>GSHMAKKPTIFILNGPNLNLLGLREPTIYGHQTLEDIANKLKLQAEKLDVTVEIRQSNHEGALIDWLQEAQAVKAKAVILNAAAYTHTSVAIYDAIRAITVPVIEVHLSNPHAREAFRHKSYVGEAALGTISGFGAESYSLALDAAAK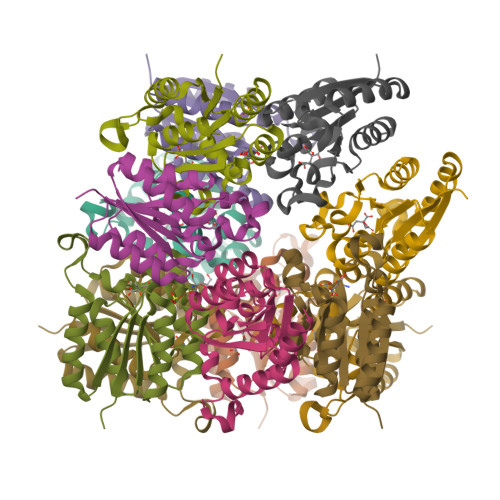L[4x]>[2x]SNAMKLGFIGLGIMGSPMAINLARAGHQLHVTTIGPVADELLSLGAVNVETARQVTEFADIIFIMVPDTPQVEDVLFGEHGCAKTSLQGKTIVDMSSISPIETKRFAQRVNEMGADYLDAPVSGGEIGAREGTLSIMVGGEQKV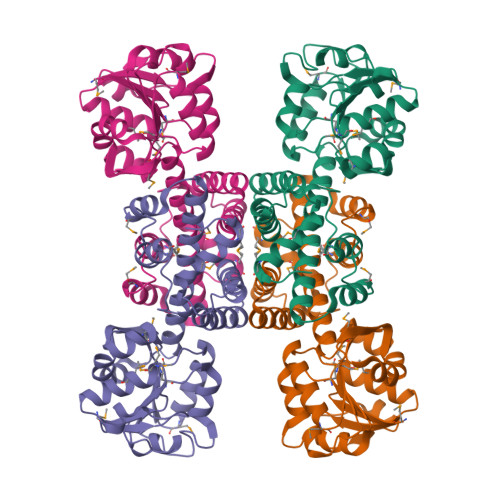FDRVKPLFDILGKNITLVGGNGDGQTCKVANQIIVALNIEAVSEALVFASKAGADPVRVRQALMGGFASSRILEVHGERMINRTFEPGFKIALHQKDLNLALQSAKALALNLPNTATCQELFNTCAANGGSQLDHSAMVQALELMANHKLS> MKIAGIDEAGRGPVIGPMVIAAVVVDENSLPKLEELKVRDSKKLTPKRREKLFNEILGVLDDYVILELPPDVIGSREGTLNEFEVENFAKALNSLKVKPDVIYADAADVDEERFARELGERLNFEAEVVAKHKADDIFPVVSAASILAKVTRDRAVEKLKEEYGEIGSGYPSDPRTRAFLENYYREHGEFPPIVRKGWKTLKKI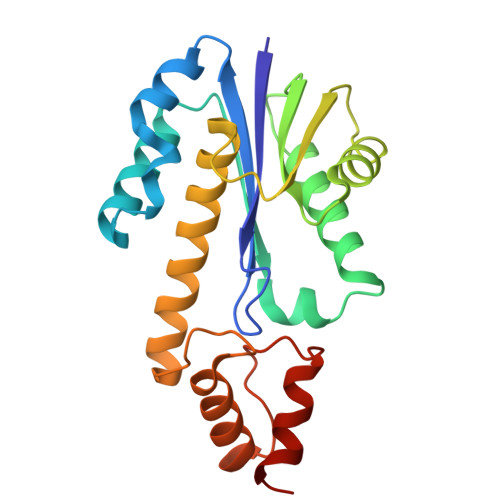TQDMINKST> MEYEWKPDEQGLQQILQLLKESQSPDTTIQRTVQQKLEQLNQYPDFN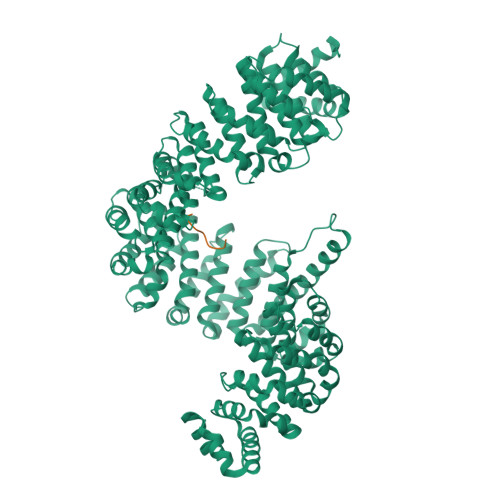NYLIFVLTKLKSEDEPTRSLSGLILKNNVKAHFQNFPNGVTDFIKSECLNNIGDSSPLIRATVGILITTIASKGELQNWPDLLPKLCSLLDSEDYNTCEGAFGALQKICEDSAEILDSDVLDRPLNIMIPKFLQFFKHSSPKIRSHAVACVNQFIISRTQALMLHIDSFIENLFALAGDEEPEVRKNVCRALVMLLEVRMDRLLPHMHNIVEYMLQRTQDQDENVALEACEFWLTLAEQPICKDVLVRHLPKLIPVLVNGMKYSDIDIILLKGDVEEDETIPDSEQDIGGSGGSGDDTISDWNLRKCSAAALDVLANVYRDELLPHILPLLKELLFHHEWVVKESGILVLGAIAEGCMQGMIPYLPELIPHLIQCLSDKKALVRSITCWTLSRYAHWVVSQPPDTYLKPLMTELLKRILDSNKRVQEAACSAFATLEEEACTELVPYLAYILDTLVFAFSKYQHKNLLILYDAIGTLADSVGHHLNKPEYIQMLMPPLIQKWNMLKDEDKDLFPLLECLSSVATALQSGFLPYCEPVYQRCVNLVQKTLAQAMLNNAQPDQYEAPDKDFMIVALDLLSGLAEGLGGNIEQLVARSNILTLMYQCMQDKMPEVRQSSFALLGDLTKACFQHVKPCIADFMPILGTNLNPEFISVCNNATWAIGEISIQMGIEMQPYIPMVLHQLVEIINRPNTPKTLLENTAITIGRLGYVCPQEVAPMLQQFIRPWCTSLRNIRDNEEKDSAFRGICTMISVNPSGVIQDFIFFCDAVASWINPKDDLRDMFCKILHGFKNQVGDENWRRFSDQFPLPLKERLAAFYGV;> SRTKRACVQKKNPLRNKQIMLRLNPY> SEKEKVEELAQRIREQLPDTELAREAQELADEARKSDDSEALKVVYLALRIVQQLPDTELAREALELAKEAVKSTDSEALKVVYLALRIVQQLPDTELARLA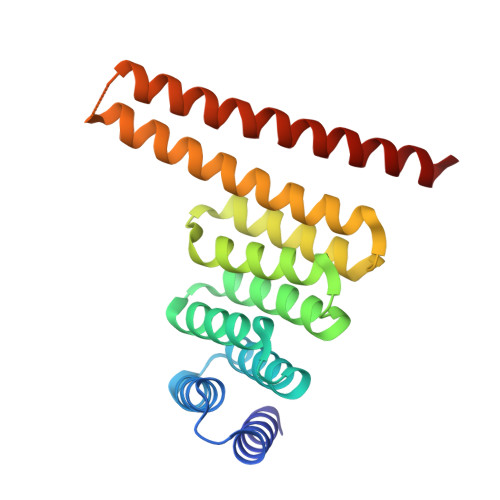LELAKKAVEMTAQEVLEIARAALKAAQAFPNTELAELMLRLAEVAARVMKELERNDEEIKKSDELDDESLLEDIVELLKEIIKLWKILVEVSDVMLKLIS> SMFKRAIIFTSFNGFEKVSRTEKRRLAKIINARVSIIDEYLRAKDTNASLDGQYRAFLFNDESP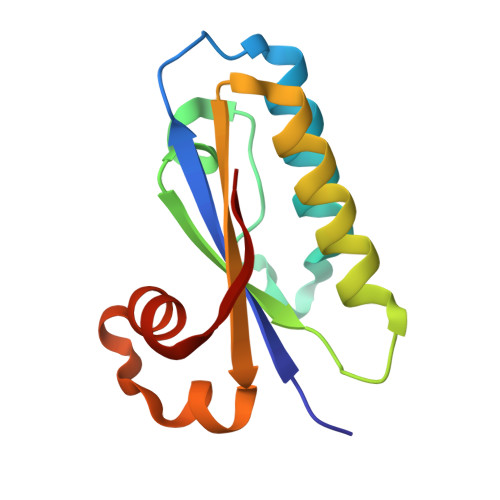AMTEFLAKLKAFAESCTGISIDAWEIEESEYVRLPVERRDFLAAANGKEIFKI> NTYQFKNMIQCTVPKRSWWDFADYGCYCGRGGSGTPIDDLDRCCQVH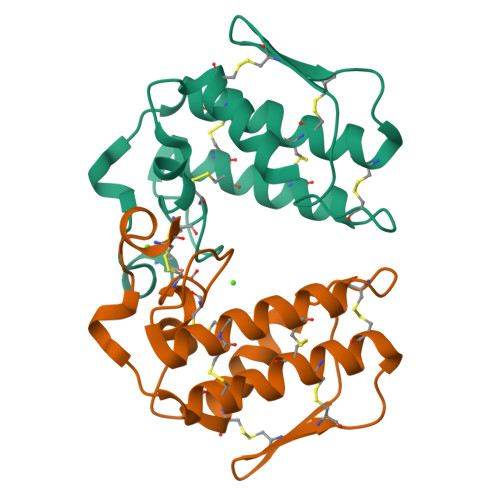DNCYNSAREQGGCRPKQKTYSYECKAGTLSCSGSNNSCAATVCDCDRLAAICFAGAPYNDNNYNIDLKARCQ;> NRWQFKNMISCTVPSRSWWDFADYGCYCGRGGSGTPVDDLDRCCQVHDNCYNEAEKISGCNPRFRTYSYECTAGTLTCTGRNNACAASVCDCDRLAAICFAGAPYNDNNYNIDLQARCN;> LVFFA>GSKKPRQKRTATKAYNVTQAFGRRGPEQTQGNFGDQELIRQGTDYKHWPQIAQFAPSASAFFGMSRIGMEV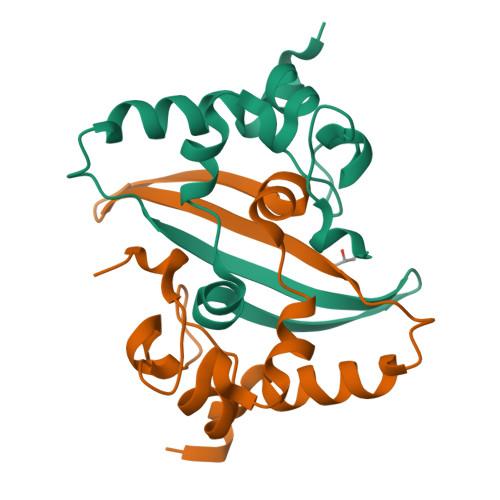TPSGTWLTYTGAIKLDDKDPNFKDQVILLNKHIDAYKTFP[8x]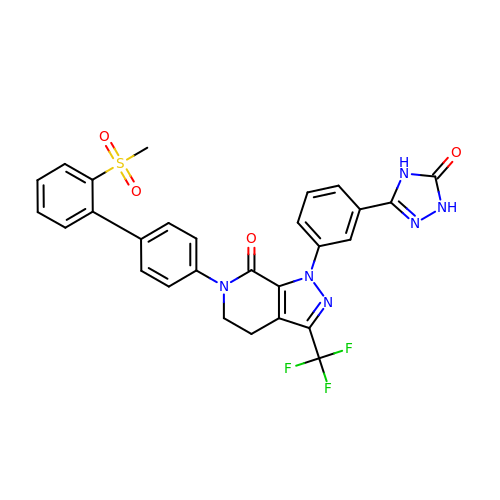6-(2'-(METHYLSULFONYL)BIPHENYL-4-YL)-1-(3-(5-OXO-4,5-DIHYDRO-1H-1,2,4-TRIAZOL-3-YL)PHENYL)-3-(TRIFLUOROMETHYL)-5,6-DIHYDRO-1H-PYRAZOLO[3,4-C]PYRIDIN-7(4H)-ONE | C28 H21 F3 N6 O4 S | LOIQROHBNJYIKB-UHFFFAOYSA-N1-[11-(dipyrrometheneboron 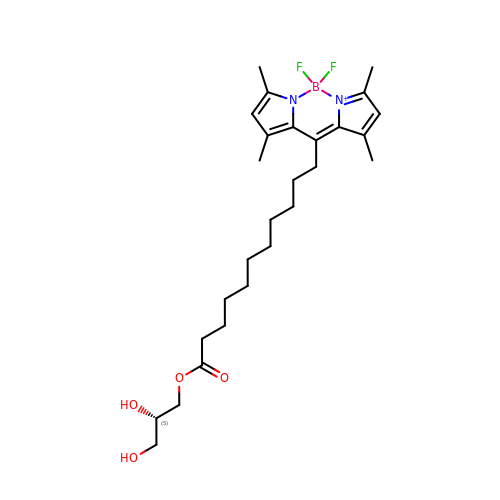difluoride)undecanoyl]-rac-glycerol | C27 H41 B F2 N2 O4 | MYLJZUQNPWUJDF-QHCPKHFHSA-N> TENLYFQ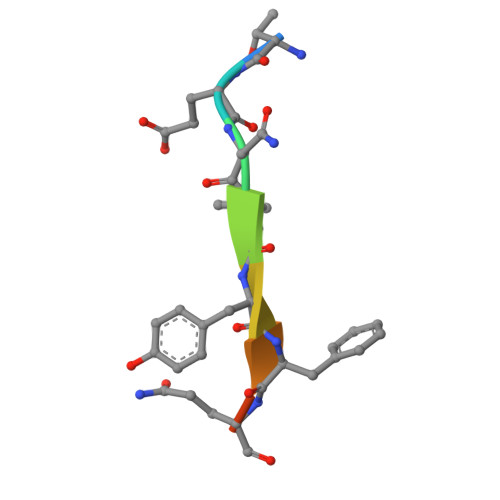GT>[6x]KLPAEFITRPHPSKDHGKETCTAYIHPNVLSSLEINPGSFCTVGKIGENGILVIARAGDEEVHPVNVITLSTTIRSVGNLILGDRLELKKAQVQPPYATKVTVGSLQGYNILECMEEKVIQKLLDDSGVIMPGMIFQNLKTKAGDESIDVVITDASDDSLPDVSQLDLNMDDMYGGLDNLFYLSPPFIFRKGSTHITFSKETQANRKYNLPEPLSYAAVGGLDKEIESLKSAIEIPLHQPTLFSSFGVSPPRGILLHGPPGTGKTMLLRVVANTSNAHVLTINGPSIVSKYLGETEAALRDIFNEARKYQPSIIFIDEIDSIAPNRANDDSGEVESRVVATLLTLMDGMGAAGKVVVIAATNRPNSVDPALRRPGRFDQEVEIGIPDVDARFDILTKQFSRMSSDRHVLDSEAIKYIASKTHGYVGADLTALCRESVMKTIQRGLGTDANIDKFSLKVTLKDVESAMVDIRPSAMREIFLEMPKVYWSDIGGQEELKTKMKEMIQLPLEASETFARLGISAPKGVLLYGPPGCSKTLTAKALATESGINFLAVKGPEIFNKYVGESERAIREIFRKARSAAPSIIFFDEIDALSPDRDGSSTSAANHVLTSLLNEIDGVEELKGVVIVAATNRPDEIDAALLRPGRLDRHIYVGPPDVNARLEILKKCTKKFNTEESGVDLHELADRTEGYSGAEVVLLCQEAGLAAIMEDLDVAKVELRHFEKAFKGIARGITPEMLSYYEEFALRS

The type II AAA + ATPase Drg1 is a ribosome assembly factor, functioning to release Rlp24 from the pre-60S particle just exported from nucleus, and its activity in can be inhibited by a drug molecule diazaborine. Here, we report Drg1 structures in different nucleotide-binding and benzo-diazaborine treated states. All structures display a typical three-layered architecture, similar to those of type II AAA + hexamers, such as p97/VCP and Cdc48, and the NTD, D1, and D2 rings show an apparent deviation from a perfect sixfold symmetry. Comparisons of these structures indicate that Drg1 hexamers transit between two extreme conformations, a planar and a helical state.

The cryo-EM map of Drg1 hexamers treated with ATP/benzo-diazaborine was resolved at a resolution of 3.8 Å (without symmetry imposed). Notably, compared with structures from other samples, this structure is more symmetrical at both the D1 and D2 rings, and the six protomers are roughly in a same conformation. While the six D2 ATPase sites in the structure of the ATP/benzo-diazaborine dataset are fully occupied by ATP, the six D2 sites in the structures from the ADP/AMPPNP/benzo-diazaborine dataset are not saturated and appear to be partially occupied by ADP. Benzo-diazaborine is docked in equivalent sites of the D1 and D2 domain. On the D1 domain, benzo-diazaborine is surround by I422, T458, R297, and R429. Importantly, benzo-diazaborine contains an extra benzyl group, which is coordinated by R429 through a cation-π interaction. Therefore, benzo-diazaborine should have also formed covalent bonds with the 2′-OH of the ribose of the ATP molecules in the ATPase centers of both the D1 and D2 domains. While the NTD and D1 remain largely as a rigid body in all these comparisons, the D2 domain of the Drg1-ATP/benzo-diazaborine complex displays a distinct conformation that is dissimilar to any of the six protomers from the mutant Drg1-ATP complex. These results suggest that benzo-diazaborine has locked the ATPase centers of Drg1 in a specific conformation and limited its conformational transition. In summary, benzo-diazaborine blocks the ATP hydrolysis cycle and hinders the conformational changes of the D1 and D2 rings, thereby disabling the conformational cycling of Drg1 subunits required for substrate processing.NLRP1 and CARD8, two related inflammasome sensors, are highly expressed in a number of cell types and play important roles in both host defense and human diseases. NLRP1 and CARD8 mediate inflammasome formation through their CARD-containing C-terminal fragment (CT) generated upon functional degradation of their respective N-terminal fragment (NT) by the proteasome. In general, inflammasomes leverage supramolecular filamentous structures to nucleate the polymerization of caspase-1, which in turn increases the local concentration of its caspase domain to facilitate dimerization and activation. Here, we determined the cryo-electron microscopy (cryo-EM) structures of NLRP1-CT and CARD8-CT filaments and analysed their assembly and specificity.

Despite being included in the construct, no UPA density was observed in the CARD8-CT cryo-EM reconstruction, which instead only reveals the central helical CARD filament. Given the predicted 17-residue unstructured linker between UPA and CARD, we proposed that UPA and any residual MBP molecules must be flexibly linked to the core CARD filament. Like other CARD filament structures, the CARD8CARD filament also possesses a one-start helical symmetry, with a refined left-handed rotation of 99.1° and an axial rise of 5.2 Å per subunit (~3.6 subunits per helical turn). The filament has a diameter of ~80 Å with a central hole of ~10 Å. In contrast, the type II interface is substantially more extensive, burying ~490 Å2 surface area per partner, and the type III interface covers ~230 Å2 per partner. Because of the small type I interface, the filament structure looks almost perforated with visible gaps. Detailed inspection of the three interfaces revealed many charge–charge pairs as well as other hydrophilic interactions including R459 at type Ia with D473 and D477 at type Ib, K509 of type IIa with D525 of type IIb, E507 of type IIa with R464 of type IIb, E479 of type IIa with Y527 of type IIb, and E483 and E487 of type IIIa with R495 of IIIb. While the wild-type protein formed filaments when the bulky MBP tag was removed, seven different point mutants, one at the type I interface, four at the type II interface, and two at the type III interface, completely abolished filament formation in vitro. CARD8CARD did not form filaments until 15 µM, while only 0.25 µM was required for CARD8UPA-CARD filament assembly, an almost 100-fold difference. In the model in which the type b surfaces of the CARD8CARD layer interact with the type a surfaces of the caspase-1CARD layer, the charge complementarity between CARD8CARD and caspase-1CARD is apparent, especially with strong negative (CARD8) and positive (caspase-1) patches both mainly at the outer rim of the filament cross-sections.

>[16x]AAFVKENHRQLQARMGDLKGVLDDLQDNEVLTENEKELVEQEKTRQSKNEALLSMVEKKGDLALDVLFRSISERDPYLVSYLRQQNL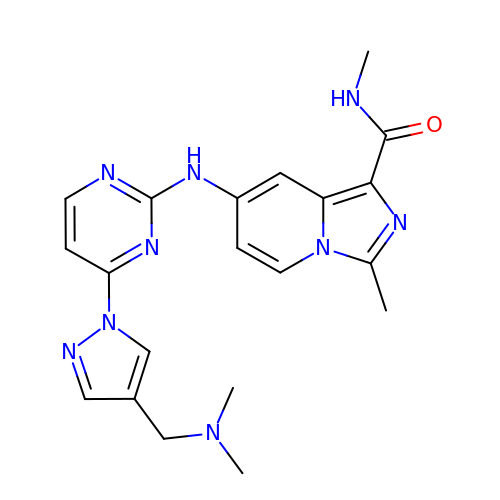7-[[4-[4-[(dimethylamino)methyl]pyrazol-1-yl]pyrimidin-2-yl]amino]-~{N},3-dimethyl-imidazo[1,5-a]pyridine-1-carboxamide | C20 H23 N9 O | PLXRPQJOIKHDDA-UHFFFAOYSA-N>AKKKATETTDEDEDGGSEKKYRKCEKAGCTATCPVCFASASERCAKNGYTSRWYHLSCGEHFCNECFDHYYRSHKDGYDKYTTWKKIWTSNGKTEPSPKAFMADQQLPYWVQCTKPECRKWRQLTKEIQLTPQIAKTYRCGMKPNTAIKPETSDHCSLPEDLRVLEVSNHWWYSMLILPPLLKDSVAAPLLSAYYPDCVGMSPSCTSTNRAAATGNASPGKLEHSKAALSVHVPGMNRYFQPFYQPNECGKALCVRPDVMELDELYEFPEYSRDPTMYLALRNLILALWYTNCKEALTPQKCIPHIIVRGLVRIRCVQEVERILYFMTRKGLINTGVLSVGADQYLLPKDYHNKSVIIIGAGPAGLAAARQLHNFGIKVTVLEAKDRIGGRVWDDKSFKGVTVGRGAQIVNGCINNPVALMCEQLGISMHKFGERCDLIQEGGRITDPTIDKRMDFHFNALLDVVSEWRKDKTQLQDVPLGEKIEEIYKAFIKESGIQFSELEGQVLQFHLSNLEYACGSNLHQVSARSWDHNEFFAQFAGDHTLLTPGYSVIIEKLAEGLDIQLKSPVQCIDYSGDEVQVTTTDGTGYSAQKVLVTVPLALLQKGAIQFNPPLSEKKMKAINSLGAGIIEKIALQFPYRFWDSKVQGADFFGHVPPSASKRGLFAVFYDMDPQKKHSVLMSVIAGEAVASVRTLDDKQVLQQCMATLRELFKEQEVPDPTKYFVT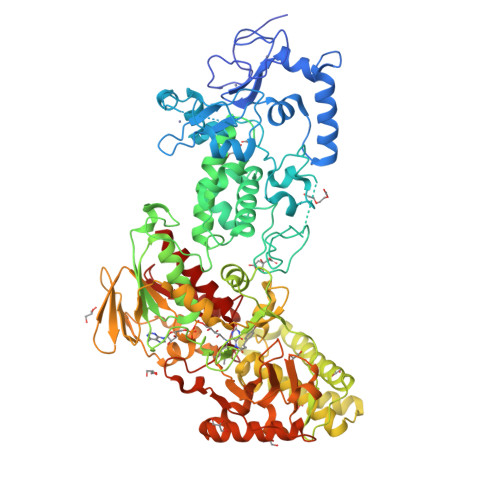RWSTDPWIQMAYSFVKTGGSGEAYDIIAEDIQGTVFFAGEATNRHFPQTVTGAYLSGVREASKIAAF[2x]> RPFIAAHFHGNTSHLNSAIHDHYKGNGLVRVSHDAPHDVWYPAPWTVASPHPRPTLTRTGHVHVHHTGVYLVYVQIYYLDSHDTISWVLHRTNADIEGRETLLQCAQSSYSTEPIDKPNSCFSAAALFLKAGDRLAVRNTAGDRHSLMQPEKSFI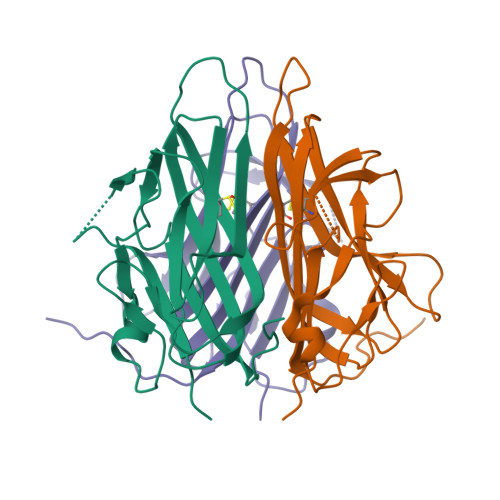GLVKLADAEDPTQEL> GPLGSMEELEQGLLMQPWAWLQLAENSLLAKVFITKQGYALLVSDLQQVWHEQVDTSVVSQRAKELNKRLTAPPAAFLCHLDNLLRPLLKDAAHPSEATFSCDCVADALILRVRSELSGLPFYWNFHCMLASPSLVSQHLIRPLMGMSLALQCQVRELATLLHMKDLEIQDYQESGATLIRDRLKTEPFEENSFLEQF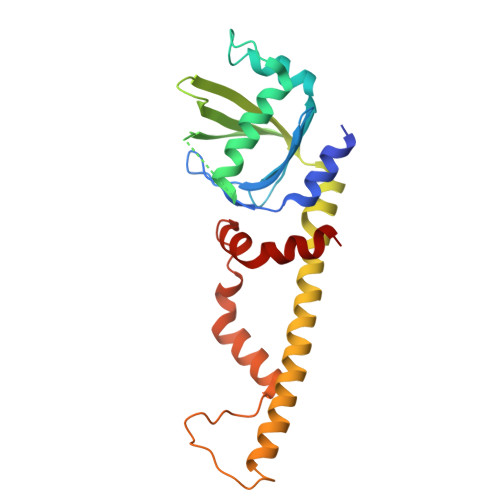MIEKLPEACSIGDGKPFVMNLQDLYMAVTTQ>[2x]GPGSMLKIALFG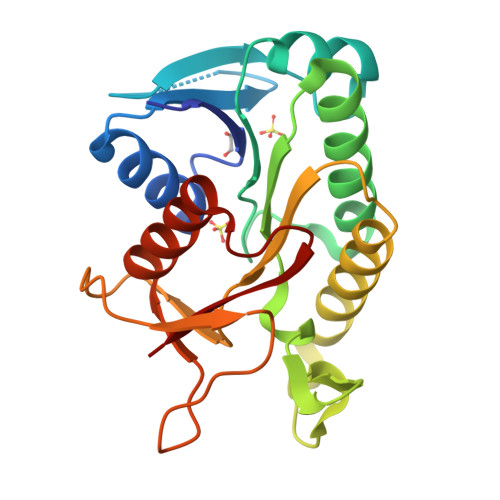ATGMIGSRIAAEAARRGHQVTALSRNPAASGANVQAKAADLFDPASIAAALAGQDVVASAYGPKQEEASKVVAVAKALVDGARKAGVKRVVVVGGAGTLEVAPGKQLVDTEGFPDAYKAVALAHRDAYGYLSTVQDLDWTFFSPAALIAPGERTGRFRTGAGRLIVDEQGNSKISAEDYAIAFVDEIEQGRFIRQAATAAY>[4x]DTLVGRADEKANERHSPQTESMITSIGNPAQVLKVRETFGTWMRESANKSDDRIWVTEHFSGIMVKEFKDLPALLNSSFTLLHLPHYFHGCGHAVYNNSLYYHKGGSNTIVRFEFGKETPQTLKLENALYFDRKYLFANSKTYFNIAVDEKGIWIIYASSVDGSSILVAQLDERTFSVTQHINTTYPKSKAGNAFIARGILYVTDTKDTRVTFAFDLLGGKQINANFDFRMSQSVLAMLSYNMRDQHLYSWEDGHLMLYPVQFLSAASSQR

Olfactomedins comprise a large protein family (PFAM: PF02191) with seven phylogenetic branches. These multidomain proteins contain a ~30 kDa olfactomedin (OLF) domain and are predominantly expressed extracellularly in a variety of tissues of multicellular organisms, particularly in vertebrates as well as selected invertebrates. Here we present biophysical, biochemical, and structural characterization of the OLF domain of a second glio-OLF, that from M. musculus (94% identical to R. norvegicus), and H. sapiens noelin/pancortin/olfm1/hOlfA (npoh-OLF), which are both neuronal OLFs, but from different phylogenetic subfamilies. The OLF domain propeller blades are arranged radially around a central hydrophilic cavity.

Gliomedin, also called collomin, collmin, and CRG-L2, is involved in the development of the peripheral nervous system and is phylogenetically most similar to invertebrate OLFs. Human and mouse glio-OLF lack these corresponding Cys residues, and the disulfide bond is replaced with a cation-π interaction involving Arg 476, at an equivalent position to Cys 409 in npoh-OLF, and Phe 541, located within the C-terminal loop immediately after strand E-21. By contrast, key amino acids present in the expected metal binding region in glio-OLF render it unable to form a coordination sphere for Ca2+. In both mouse and rat glio-OLF structures, an apparent Na+ ion is coordinated by Asn 423, Asn 471, Ala 472, Leu 517, and a water molecule. In our structure, this ion assignment was made based on lack of stabilization by Ca2+, Mg2+, or K+ in solution, unresponsiveness to Quin-2, fit of electron density, and refined metal-ligand distances consistent with Na+. In glio-OLF, analogous residues to the Trp/Tyr pair are Asn 417/Asp 486, which are hydrogen bonded; this cross-loop interaction is further stabilized by hydrogen bonding between Asn 417 and the main chain carbonyl oxygen of Thr 484 on loop D-16/D-17. Thus, the available glio-OLF structures appear to be in a closed conformation that prevents access to the central cavity. Comparison of hydrophobic interactions among glio-OLF, npoh-OLF, and myoc-OLF reveals at least 20 more hydrophobic interactions for glio-OLF.> EEDCWKNEELKEDCVGPLIAPKDCTDKDHKTYLSEASLLATAKKITQVDAENVEILGKTMESAIRVIERQKTYHRMHLLEAVFLNKHCDYYKMFEHNSGYSQVKWRMMIKTQHFDICALQANSPFCAQCIADNSCAQGSWEFDTHMNSTYSSKVDNFKHDFSLFLRIFEAAFPGTAYVHLLTNIKEKKPYQAVSMIEKIKKKFPNNKLLIGYLDFGKYLLGLSHASTYELQQRQLDKLYQPTELGGWSHPQFEK

The OBV M segment encodes two glycoproteins, Gn and Gc, derived from a single polyprotein precursor, with Gn encoded upstream of Gc. Compared with other bunyaviruses, OBV Gn is relatively small, with an ectodomain of about 200 amino acids (aa), whereas Gc, with an ectodomain of ca. 900 aa long, is about twice the size of its Gc counterparts from other bunyaviruses. Our structural analysis has revealed that this region is composed of two domains: a 27 -kDa α-helical head domain and a stalk that is divided into two identically folded 19 -kDa tandem β-sandwiches. Furthermore, the head domain is well exposed to the environment and is a major target of the humoral adaptive immune system of the OBV mammalian hosts, indicating that the trigonal pyramid of the spike shields the functionally more critical membrane fusion core machinery from the host’s antibody response.

In addition to the variable region of SBV Gc, we determined the crystal structures of the Gc head domains from BUNV (aa 478–721), LACV (aa 477–722) and OROV (aa 482–702) to resolutions ranging between 2.1 Å and 2.9 Å and refined the resulting atomic models to Rfree values between 0.21 and 0.23. The head domains of BUNV, LACV, and OROV contain each a single asparagine-linked carbohydrate chain and although the positions of the respective glycosylation sites along the aa sequences are not conserved, they project from the same face of the domain carrying the two glycan chains in SBV. Nevertheless, the Gc head domains of BUNV and LACV both formed trimeric assemblies involving the same trimerization contacts in the crystals. The buried surface area at the trimer interface amounts to 1422 Å2 and 1430 Å2 on each protomer for BUNV and LACV, respectively. Whereas the atomic details at these interfaces differ between the two viruses, they comprise mainly hydrophilic residues in the region between helices h7 and h11 at the side opposite to the glycosylated surface. The concurrent observation of two very similar trimeric assemblies in two independent crystal structures strongly suggests that the trimers are physiologically relevant. While the low resolution of this reconstruction does not allow for a sequence-correlated domain assignment per se, our crystal structure of the trimeric BUNV Gc head domain fits unambiguously into the most membrane-distal region of this pyramid (correlation coefficient = 0.92). Consequently, the three legs of the tripodal pyramid must each accommodate the stalk (correlation coefficient = 0.88). The dissociation of the trimers at low pH is likely triggered by protonation of residue H590 in BUNV and in LACV, which would lead to electrostatic repulsion with positively charged side chains on the neighboring protomer.> GSNVNKIYIENHDLMSKVPVIEASKESTRDDWAALTVVADLDDIEGQELVYYALRFRKS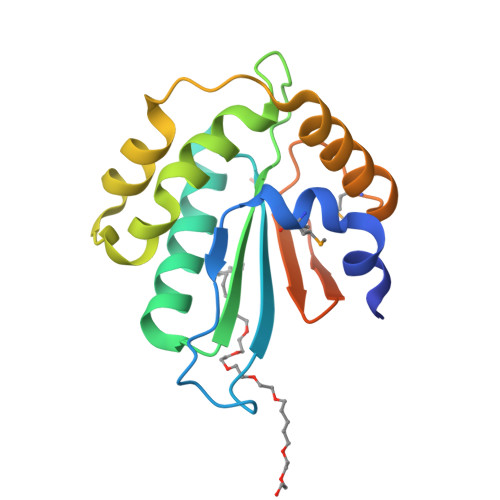NDGVRLDIVHNPKDTSRSPSVLAQRLKSREDKLLDFTRFLDLETALETGEFEPDVAYDASLANFLASSNMKAGDNFVILNGRVLGPITSADDFKKEDFEVFLQA> CLAEGTRIFDPVTGTTHRIEDVVGGRKPIHVVAAAKDGTLH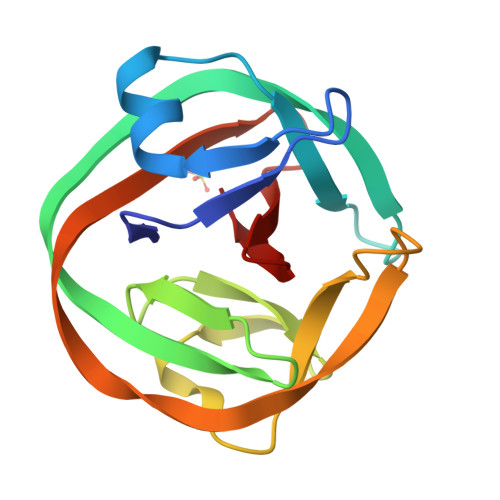ARPVVSWFDQGTRDVIGLRIAGGAILWATPDHKVLTEYGWRAAGELRKGDRVAVRDVETGELRYSVIREVLPTRRARTFGLEVEELHTLVAEGVVVHN>[2x]SEKITDGINKTISATGNIYNISSANELNALKLQPGDKVIFKKGNWKNQQINFKANGTKEKPVVLAAEKGGETIFSGNSNLKIDGNWLVVDGFVFKDGFSEKADVILFTKSTSNSRITNSSIINYNHPDKTFDYKWLSLNGENNRVDHCDFTGKTHQGTTLVVWLDEKPNHHQIDHNYFGPRPALGVNGGETIRIGTSTWSMHDSYTLVENNIFDKCDGEMEIISLKSGHNTVNNNLFYECDGT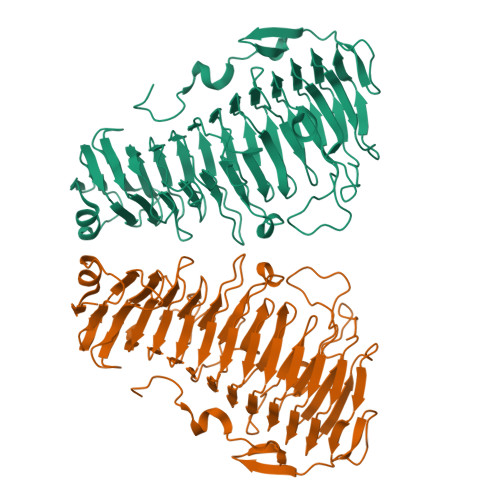VTFRHGNYNTVSNNYILGNGKKNTGGIRIIGENHKVFGNYLQGLDGSGLRAAISIMSALEKPQLHEYFQVINPQIVGNIIADSKEGIDIGAGKNEKRMLPPKDGFLKNNYVINTRTVIKTENEPEGLLIENNQTDASSLPKGFTKVGSDLVKSDGIWQKKNDVKTPFWKKEKIGPEWNNVKMNF> SYYRSINAADLYENIKAYTVLDVREPFELIFGSIANSINIPISELREKW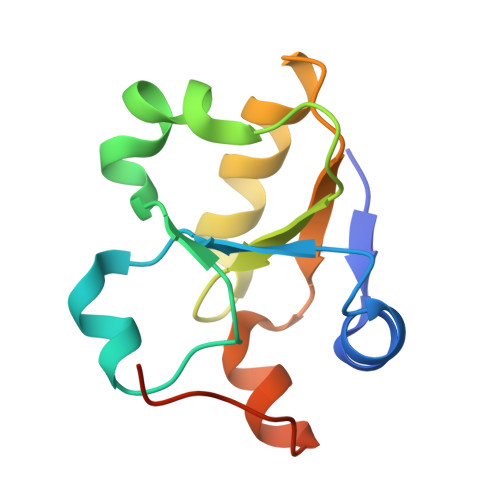KILERDKKYAVICAHGNRSAAAVEFLSQLGLNIVDVEGGIQSWIEEGYPVVLEHHHHHH> FLATTLERIEKNFVITDPRLPDNPIIFASDSFLQLTEYSREEILGR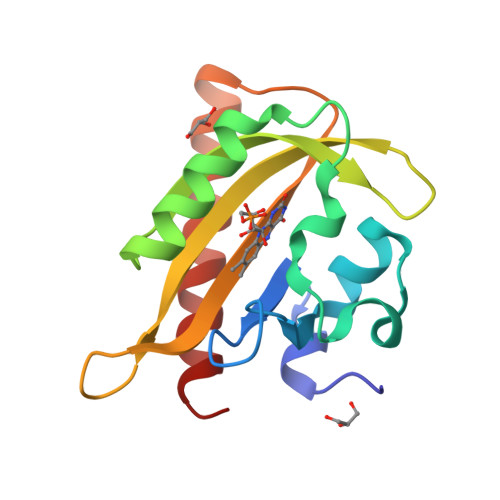NCRFLQGPETDRATVRKIRDAIDNQTEVTVQLINYTKSGKKFWNLFHLQPMRDQKGDVQYFIGVQLDGTEHVRDAAEREGVMLIKKTAENIDEAAKEL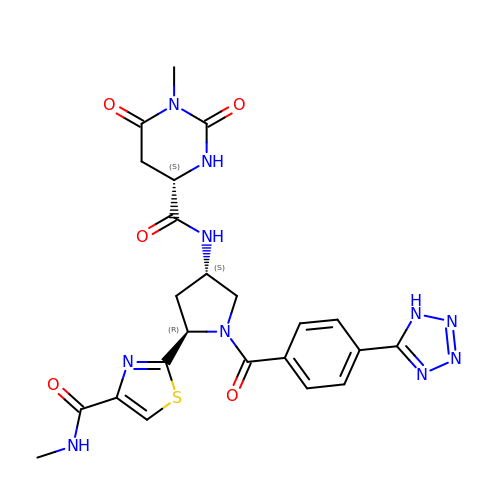(4S)-1-methyl-N-{(3S,5R)-5-[4-(methylcarbamoyl)-1,3-thiazol-2-yl]-1-[4-(1H-tetrazol-5-yl)benzene-1-carbonyl]pyrrolidin-3-yl}-2,6-dioxohexahydropyrimidine-4-carboxamide | C23 H24 N10 O5 S | SYFLGRBSBZONAM-OFQRWUPVSA-N>GSAVPFHGAHQAGIATPVQDRLHFAAFDVTTEDRAAFVALLKEWTAAARRLTAGHAVGEGAYGGLPEAPPDDTGEALGLKPSRLTLTIGFGPSLFTRFGLADLRPEALADLPKFPGDNLDRARSGGDLCVQACADDPQVAVHAIRNLARIGFGKVVVRWSQLGFGKTSSTTPDKQTPRNLLGFKDGTRNIAGTEKDRLDRFVWAAEKDGTPWMTGGSYLVARRIRMHIETWDRASLQEQEDVFGRDKGEGAPVGKAKERDEPFLKAMKPDAHVRLAHPDSNGGATLLRRGYSFTDGTDGLGRLDAGLFFLAYQRDIRT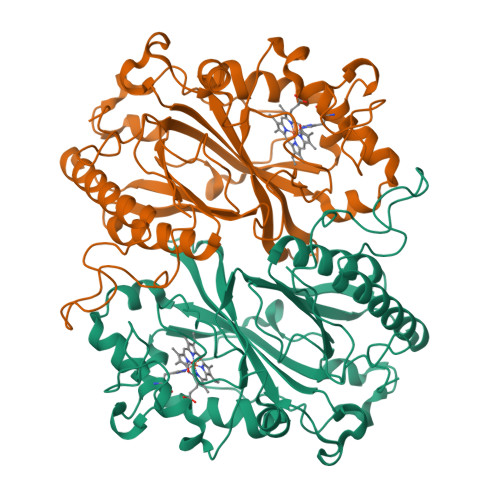GFVPVQRNLATDALNEYIQHVGSAVFAVPPGVRDADDWWGSTLF[2x]>[2x]GPGSTSAVLLDHCHFSQVIFNSVEKFYIPGGDVTCHYTFTQHFIPRRKDWIGIFRVGWKTTREYYTFMWVTLPIDLNNKSAKQQEVQFKAYYLPKDDEYYQFCYVDEDGVVRGASIPFQFRPENEEDILVVTTQGE;>[2x]GSEFSLVAELQEKLQEEKAKFLEQLEEQEKRKNEEMQNVRTSLIAEQQTNFNTVLTREKMRKENIINDLSDKLKSTM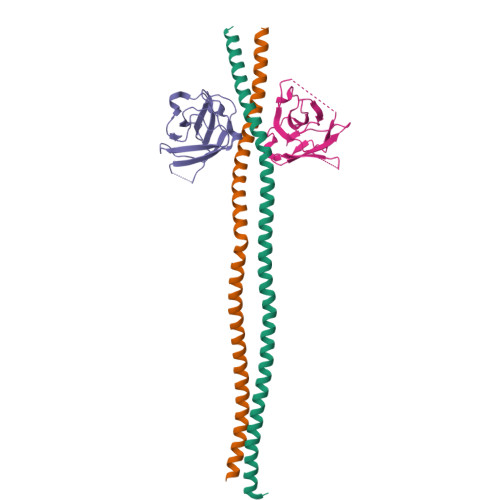QQQERDKDLIESLSEDRARLLEEKKKLEEEVSKLRSS>[2x]GSDDDNPTVDPANIDYTPENASSWHNYMRNVAALLKTDATNLYNAWNSSYKGGESYASLFKAHSGSPYASALSCVEEIVDKCAEIANEVGTAKIGDPYNLYKAGNTEEALYAVESWYSWHSRDDYTNNIYSIR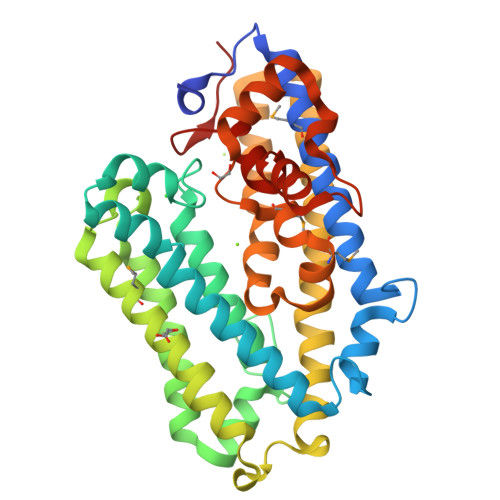NAYYGSLDGNINANSLSTVIAGANSSLDTKIKNAIQKAAKAIQDIPQPFRNHIPSNETVAAMDACAELESILKNDLKSYIANNSNNINTDAVLNPVVTQYVDAVVVPTYKSLKEKNDALYNAVIVLADNPSNSAFETACDAWITAREPWEKSEAFLFGPVDEMGLDPNMDSWPLDQNAIVQILNSQSWSDLEWSEGDDEAAVESAQNVRGFHTLEFLLYKNGEPRKVQ> ELVLALYDYQEKSPREVTMKKGDILTLLNSTNKDWWKVEVND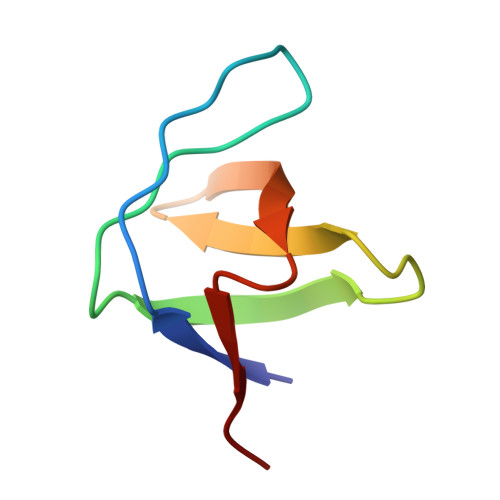RQGFVPAAYVKKLD> HPETLVKVKDAEDQLGARVGYIELDLNSGKILESFRPEERFPMMSTFKVLLCGAVLSRIDAGQEQLGRRIHYSQNDLVAASPVTEKHLTDGMTVRELCSAAI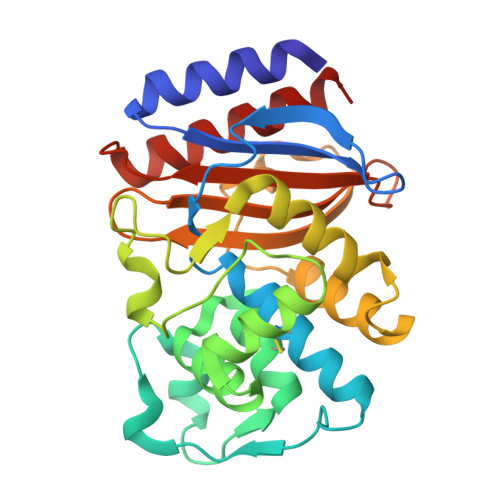TMSDNTAANLLLTTIGGPKELTAFLHNMGDHVTRLDRWEPELNEAIPNDERDTTMPAAMATTLRKLLTGELLTLASRQQLIDWMEADKVAGPLLRSALPAGWFIADKSGAGERGSRGIIAALGPDGKPSRIVVIYTTGSQATMDERNRQIAEIGASLIKHW> MSTPPLAPTGMASGPFGGPQAQQAAREVNTATLCRIGQETVQDIVYRTMEIFQLLRNMQLPNGVTYHTGTYQDRLTKLQDHLRQLSILFRKLRLVYDKCNENCGGMDPIPVEQLIPYVDEDGSKNDDRAGPPRF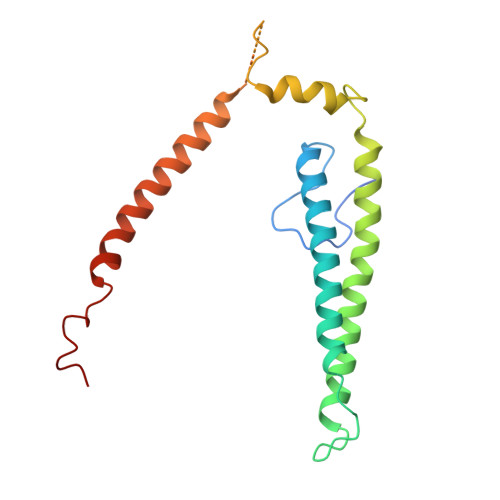ASEERREIVEVNKKLKQKNQQLKQIMDQLRNLIWDINAMLAMRN> MDYDELLKYYELHETIGTGGFAKVKLACHILTGEMVAIKIMDKNTLGSDLPRIKTEIEALKNLRHQHICQLYHVLE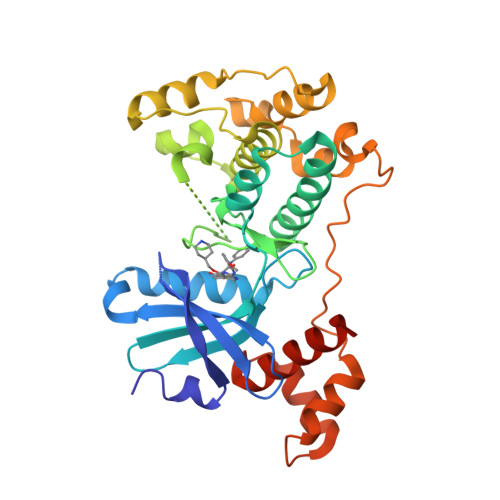TANKIFMVLEYCPGGELFDYIISQDRLSEEETRVVFRQIVSAVAYVHSQGYAHRDLKPENLLFDEYHKLKLIDFGLCAKPKGNKDYHLQTCCGSLAYAAPELIQGKSYLGSEADVWSMGILLYVLMCGFLPFDDDNVMALYKKIMRGKYDVPKWLSPSSILLLQQMLQVDPKKRISMKNLLNHPWIMQDYNYPVEWQSKNPFIHLDDDCVTELSVHHRNNRQTMEDLISLWQYDHLTATYLLLLAKKARGKPVHHHHHH> GLDTLDRDGDGSTADADCN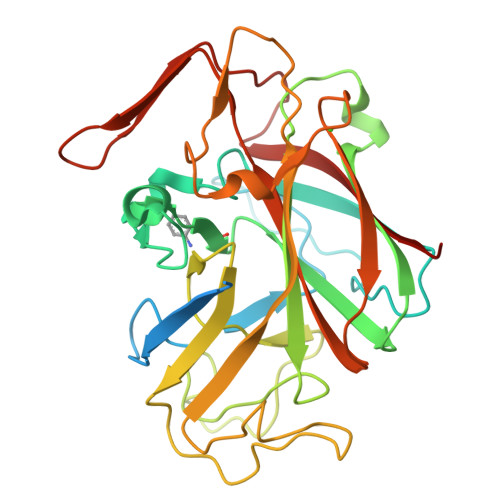DFAPTIHPGAAEATLDGVDSNCDGRDSGVAEVVETFKNPGTYSSPVINFKIASPPGPGTPIYGPPRDFSGYNKSYSLAIGKTSYYDPTTGTKWNDDTITPVSDGQDIWRGWTHTGKWSFFNGKAGDKITLSVQRDAQEASLKGAHPGFILFWRPEGGPLFWAGTQDLDEGQTALPADSDTVIGHVIVQHADWTLQGLPPKADHTAPAGVDTELYPMKPDSYTMYYVDSGYDADKYVASKKLIMHPTAFKGLALNDGTAGAFTKSITLPKTGYYMLYVANVLEVDDWSVDADGKLTTTGEVWEVPAKGCWVNITISKP> MSGLRTVSASSGNGKSYDSIMKILLIGDSGVGKSCLLVRFVEDKFNPSFITTIGIDFKIKTVDINGKKVKLQLWDTAGQERFRTITTAYYRGAMGIILVYDVTDERTFTNIKQWFKTVNEHANDEAQLLLVGNKSDMETRVVTADQGEALAKELGIPFIESSAKNDDNVNEIFFTLAKLIQEKIDSNKLVGVGNGKEGNISINSGSGNSSKSN;>[2x]MDQETIDTDYDVIVLGTGITECILSGLLSVDGKKVLHIDKQDHYGGEAASVTLSQLYEKFKQNPISKEERES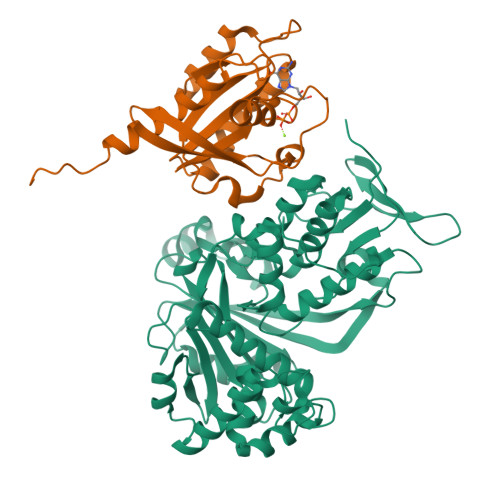KFGKDRDWNVDLIPKFLMANGELTNILIHTDVTRYVDFKQVSGSYVFKQGKIYKVPANEIEAISSPLMGIFEKRRMKKFLEWISSYKEDDLSTHQGLDLDKNTMDEVYYKFGLGNSTKEFIGHAMALWTNDDYLQQPARPSFERILLYCQSVARYGKSPYLYPMYGLGELPQGFARLSAIYGGTYMLDTPIDEVLYKKDTGKFEGVKTKLGTFKAPLVIADPTYFPEKCKSTGQRVIRAICILNHPVPNTSNADSLQIIIPQSQLGRKSDIYVAIVSDAHNVCSKGHYLAIISTIIETDKPHIELEPAFKLLGPIEEKFMGIAELFEPREDGSKDNIYLSRSYDASSHFESMTDDVKDIYFRVTGHPLVLKQRQEQEKQ>[12x]MKQLATPFQEYSQKYENIRLERDGGVLLVTVHTEGKSLVWTSTAHDELAYCFHDIACDRENKVVILTGTGPSFCNEIDFTSFNLGTPHDWDEIIFEGQRLLNNLLSIEVPVIAAVNGPVTNAPEIPVMSDIVLAAESATFQDGPHFPSGIVPGDGAHVVWPHVLGSNRGRYFLLTGQELDARTALDYGAVNEVLSEQELLPRAWELARGIAEKPLLARRYARKV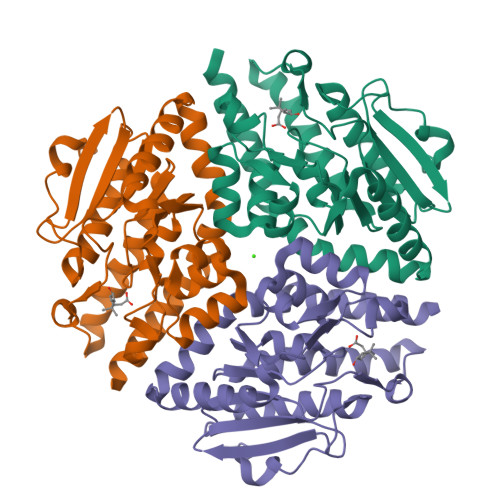LTRQLRRVMEADLSLGLAHEALAAIDLGMESEQ> PKDAQVIMSILKELNVQEYEPRVVNQLLEFTFRYVTSILDDAKVYANHARKKTIDLDDVRLATEVTLD;> MLYGS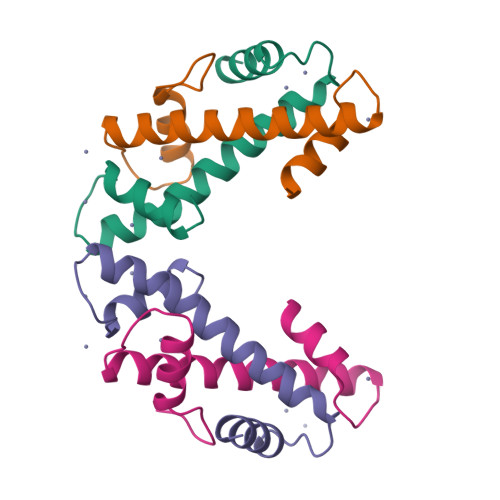SISAESMKVIAESIGVGSLSDDAAKELAEDVSIKLKRIVQDAAKFMNHAKRQKLSVRDIDMSLKV> LEDPGEGQDIWDMLDKGNPFQFYLTRVSGVKPKYNSGALHIKDIL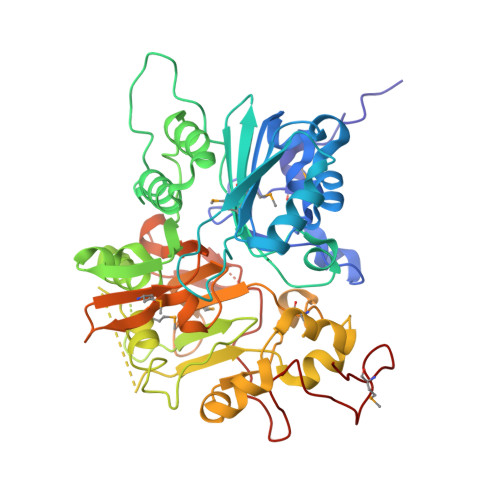SPLFGTLVSSAQFNYCFDVDWLVKQYPPEFRKKPILLVHGDKREAKAHLHAQAKPYENISLCQAKLDIAFGTHHTKMMLLLYEEGLRVVIHTSNLIHADWHQKTQGIWLSPLYPRIADGTHKSGESPTHFKANLISYLTAYNAPSLKEWIDVIHKHDLSETNVYLIGSTPGRFQGSQKDNWGHFRLKKLLKDHASSMPNAESWPVVGQFSSVGSLGADESKWLCSEFKESMLTLGKESKTPGKSSVPLYLIYPSVENVRTSLEGYPAGGSLPYSIQTAEKQNWLHSYFHKWSAETSGRSNAMPHIKTYMRPSPDFSKIAWFLVTSANLSKAAWGALEKNGTQLMIRSYELGVLFLPSALGLDSFKVKQKFFAGSQEPMATFPVPYDLPPELYGSKDRPWIWNIPYVKAPDTHGNMWVPS> GPLGSMAQGTLIRVTPEQPTHAVCVLGTLTQLDICSSAPEDCTSFSINASPGVVVDIAHSPPAKKKSTGSSTWPLDPGVEVTLTMKAASGSTGDQKVQISYYGPKTPPVKALLYLTAVEISLCADITRTGKVKPTRAVKDQRTWTWGPCGQGAILLVNCDRDNLESSAMDCEDDEVLDSEDLQDMSLMTLSTKTPKDFFTNHTLVLHVARSEMDKVRVFQATRGKLSSKCSVVLGPKWPSHYLMVPGGKHNMDFYVEALAFPDTDFPGLITLTISLLDTSNLELPEAVVFQDSVVFRVAPWIMTPNTQPPQEVYACSIFENEDFLKSVTTLAMKAKCKLTICPEEENMDDQWMQDEMEIGYIQAPHKTLPVVFDSPRNRGLKEFPIKRVMGPDFGYVTRGPQTGGISGLDSFGNLEVSPPVTVRGKEYPLGRILFGDSCYPSNDSRQMHQALQDFLSAQQVQAPVKLYSDWLSVGHVDEFLSFVPAPDRKGFRLLLASPRSCYKLFQEQQNEGHGEALLFEGIKKKKQQKIKNILSNKTLREHNSFVERCIDWNRELLKRELGLAESDIIDIPQLFKLKEFSKAEAFFPNMVNMLVLGKHLGIPKPFGPVINGRCCLEEKVCSLLEPLGLQCTFINDFFTYHIR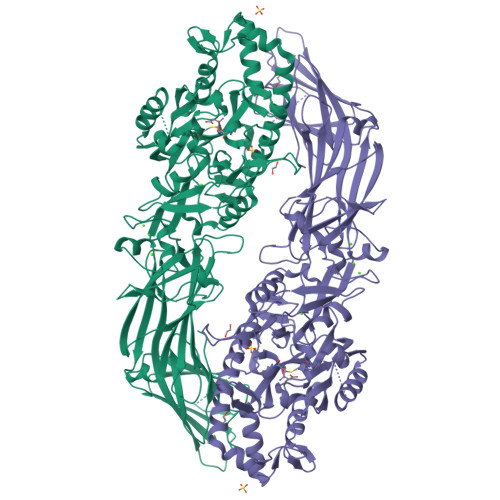HGEVHCGTNVRRKPFSFKWWNMVP>SLRANDAPIVLLHGLTGWGREEMFGFKYWGGVRGDIEQWLNDNGYRTYTLAVGPLSSNWDRACEAYAQLVGGTVDYGAAHAAKHGHARFGRTYPGLLPELKRGGRIHIIAHSQGGQTARMLVSLLENGSQEEREYAKAHNVSLSPLFEGGHHFVLSVTTIATPHDGTTLVNMVDFTDRFFDLQKAVLEAAAVASNVPYTSQVYDFKLDQWGLRRQPGESFDHYFERLKRSPVWTSTDTARYDLSVSGAEKLNQWVQASPNTYYLSFSTERTYRGALTGNHYPELGMNAFSAVVCAPFLGSYRNPTLGIDDRWLENDGIVNTVSMNGPKRGSSDRIV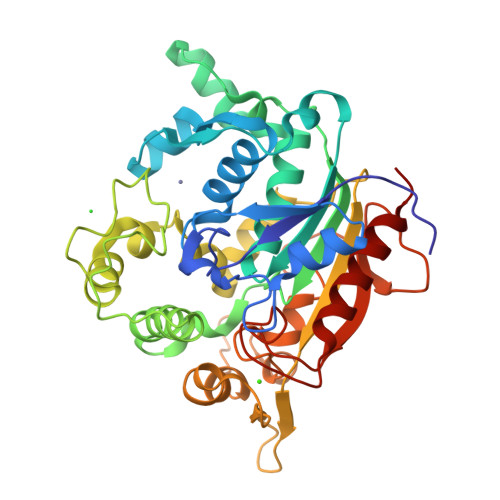PYDGTLKKGVWNDMGTYNVDHLEIIGVDPNPSFDIRAFYLRLAEQLASLQP[2x]>ADTKEVLEAREAYFKSLGGSMKAMTGVAKAFDAEAAKVEAAKLEKILATDVAPLFPAGTSSTDLPGQTEAKAAIWANMDDFGAKGKAMHEAGGAVIAAANAGDGAAFGAALQKLGGTCKACHDDYRE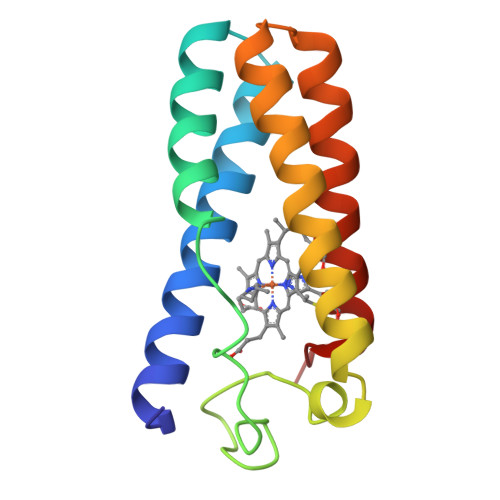ED[2x]phosphinate 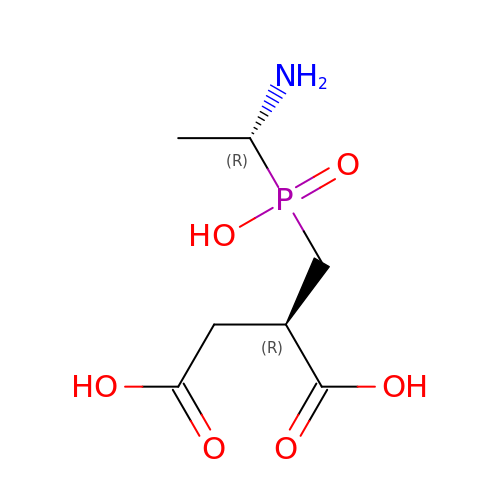pseudodipeptide L-Ala-D-Asp | C7 H14 N O6 P | LWODXTSWCZWQHR-UHNVWZDZSA-N> UGCUCCUAGUACGAGAGGACXGGAGUG

To this end, we used the 27 nt fragment of E. coli 23 S rRNA sarcin-ricin loop (SRL) region. This sequence is known to be a robust and well-behaved crystallization scaffold that can accommodate small modifications. For the installation of 2′-OCF3, we deemed nucleotide A2670 appropriate which forms a Watson−Crick base pair with U2650 in the regular A-form double helical region of this RNA, as well as nucleotide C2667 which forms a water-mediated mismatch with U2653. The study is complemented by crystal structures of an RNA hairpin including 2′-OCF3 modifications.

The study is complemented by a crystal structure at 0.9 Å resolution of a 27 nt hairpin RNA containing a single 2′-OCF3 group that well integrates into the minor groove. As previously observed for the 2′-SCF3–C2667 modification, a fluorine atom of the 2′-OCF3 group closely approached the oxygen atom of its cytosine nucleobase (O2). It is tempting to assume that the short distance observed (2.9 Å) is indicative of a halogen bond, however, fluorine (as opposed to chlorine, bromine, or iodine) usually retains a strongly electronegative electrostatic potential in biomolecules.> MGHHHHHHENLYFQGVQKIGILGAMREEITPILELFGVDFEEIPLGGNVFHKGVYHNKEIIVAYSKIGKVHSTLTTTSMILAFGVQKVLFSGVAGSLVKDLKINDLLVATQLVQHDVDLSAFDHPLGFIPESAIFIETSGSLNALAKKIANEQHIALKEGVIASGDQFVHSKERKEFLVSEFKASAVEMEGASVAF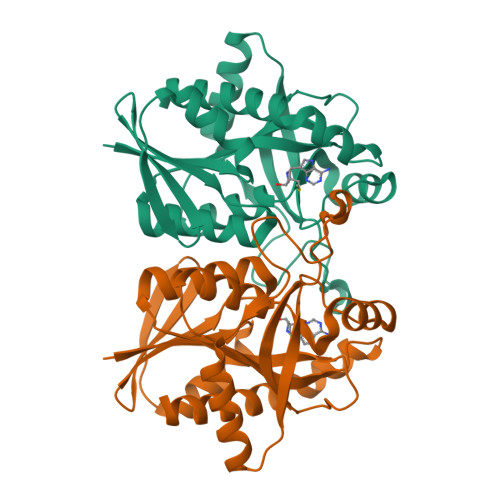VCQKFGVPCCVLRSISDNADEKAGMSFDEFLEKSAHTSAKFLKSMVDEL The human Merkel cell polyomavirus (MCPyV or MCV) was discovered in 2008 and found to be clonally integrated into Merkel cell carcinomas (MCCs), establishing it as the first human oncovirus from the polyomavirus family. Polyomavirus infectious entry is initiated by the major capsid protein VP1, which attaches to cellular receptors to promote internalization and transport of the viral genome into the nucleus for replication. MCPyV VP1 is a symmetric ring-shaped homopentamer with the five VP1 monomers arranged around a central five-fold axis. Each monomer is composed of two antiparallel β-sheets, which together form a β-sandwich with jelly-roll topology.

We solved the crystal structure of unassembled MCPyV VP1 pentamers at 2.1 Å resolution. The crystallized VP1 construct was truncated at the C-terminus to prevent VP1 assembly into capsids, and at the N-terminus to remove potentially disordered residues that inhibit crystallization. However, the construct contained the entire pentameric core of VP1. Similar truncations did not have an effect on the receptor binding properties of other polyomavirus VP1 proteins. With β-strands named alphabetically from the N-terminus, the two sheets consist of strands B, I, D, G, and C, H, E, F, respectively. The β-strands are linked by extensive loops that cover the top and sides of the pentamer. The apical loops, which make up the top surface of the pentamer and thus the outer surface of the virus, are the most variable parts among VP1 sequences from different polyomaviruses, creating unique interaction surfaces. The structure of MCPyV VP1 bound to the oligosaccharides is virtually identical to the unbound state, indicating that the carbohydrates dock into a preformed binding pocket.

>[20x]GSHMLEGGVEVLSVVTGEDSITQIELYLNPRMGVNSPDLPTTSNWYTYTYDLQPKGSSPDQPIKENLPAYSVARVSLPMLNEDITCDTLQMWEAISVKTEVVGISSLINVHYWDMKRVHDYGAGIPVSGVNYHMFAIGGEPLDLQGLVLDYQTQYPKTTNGGPITIETVLGRKMTPKNQGLDPQAKAKLDKDGNYPIEVWCPDPSKNENSRYYGSIQTGSQTPTVLQFSNTLTTVLLDENGVGPLCKGDGLFISCADIVGFLFKTSGKMALHGLPRYFNVTLRKRWVKN> MADVAGTSNRDFRGYILSVQAEEQKNYNNSLNGEVSVWVYAYYSDGSVLVINKNSQYKVGISETFKALKEYREGQHNDSYDEYEVNQSIYYPNGGDARKFHSNAKPRAIQIIFSPSVNVRTIKMAKGNAVSVPDEYLQRSHPWEATGIKYRKIKRDGEIVGYSHYFELPHEYNSISLAVSGVHKNPSSYNVGSAHNVMDVFQSCDLALRFCNRYW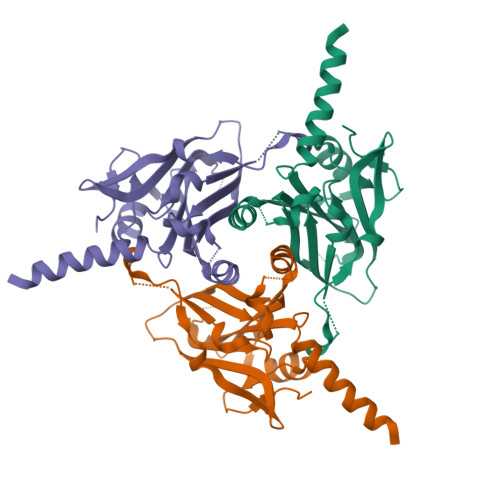AELELVNHYISPNAYPYLDINNHSYGVALSNRQ>[2x]MGHHHHHHKVNEVSWSDLEQEVAQA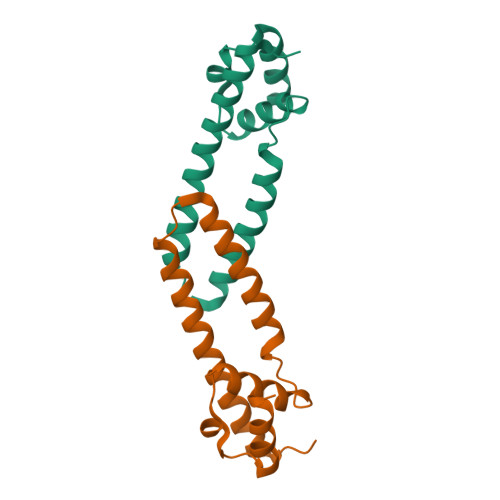AFQKAYEREINALIQDVRDNAVQISELEDIWRLHNFLSAKRHEIDGKYDYNYSVLVFVFATLIKQGWLHLDELKGLDQDKLTKIGSLSRM>[4x]MHGSNKLPGFATRAIHHGYDPQDHGGALVPPVYQTATFTFPTVEYGAACFAGEQAGHFYSRISNPTLNLLEARMASLEGGEAGLALASGMGAITSTLWTLLRPGDEVLLGNTLYGCTFAFLHHGIGEFGVKLRHVDMADLQALEAAMTPATRVIYFESPANPNMHMADIAGVAKIARKHGATVVVDNTYCTPYLQRPLE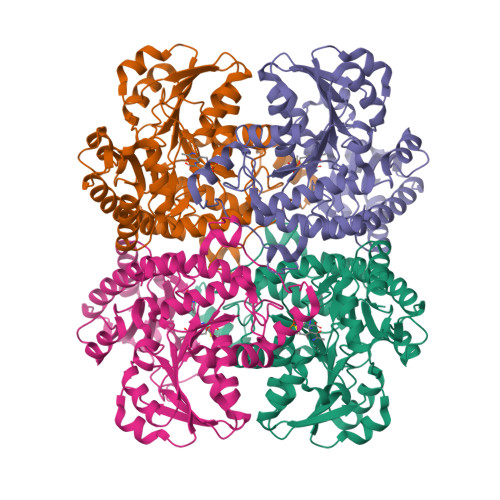LGADLVVHSATKYLSGHGDITAGIVVGSQALVDRIRLQGLKDMTGAVLSPHDAALLMRGIKTLNLRMDRHCANAQVLAEFLARQPQVELIHYPGLASFPQYTLARQQMSQPGGMIAFELKGGIGAGRRFMNALQLFSRAVSLGDAESLASHPASMTHSSYTPEERAHYGISEGLVRLSVGLEDIDDLLADVQQALKASA(3S)-2,2-dimethyl-3,4-dihydro-2H-1,4-thiazine-3,6-dicarboxylic acid | C8 H11 N O4 S | 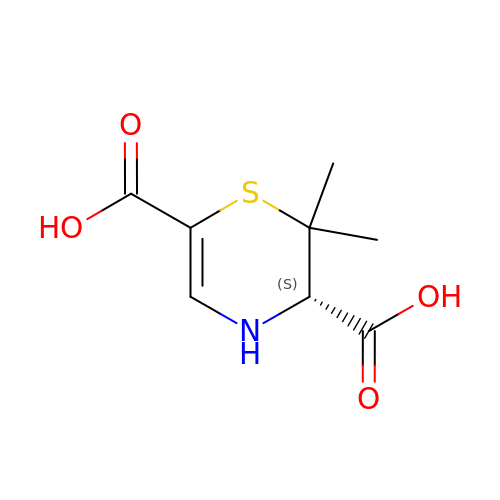VSZLPINYHQLOJH-YFKPBYRVSA-N N-ACETYL-SERINE | C5 H9 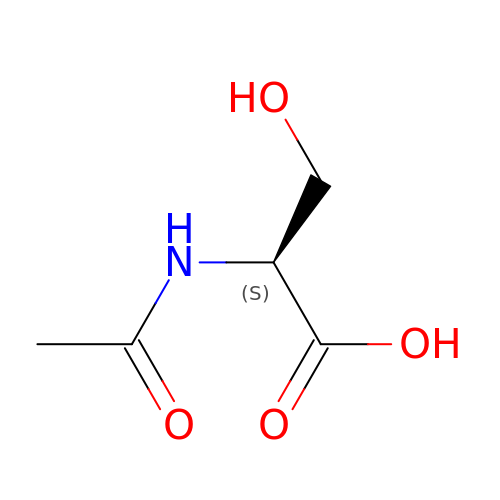N O4 | JJIHLJJYMXLCOY-BYPYZUCNSA-N> MDLSQLTPRRPYLLRAFYEWLLDNQLTPHLVVDVTLPGVQVP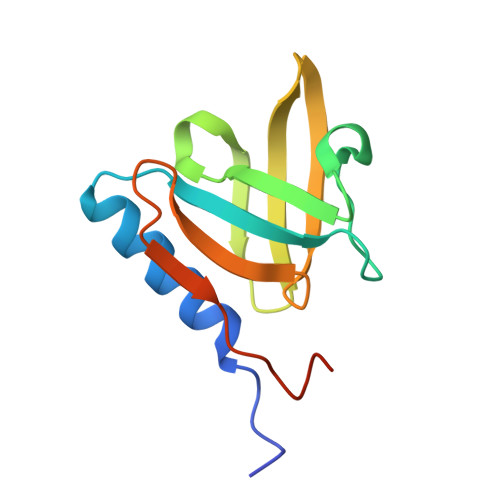MEYARDGQIVLNIAPRAVGNLELANDEVRFNARFGGIPRQVSVPLAAVLAIYARENGAGTMFEPEAAYDEDTSIMN The yeast diadenosine and diphosphoinositol polyphosphate phosphohydrolase DDP1 is a Nudix enzyme with pyrophosphatase activity on diphosphoinositides, dinucleotides, and polyphosphates. ScDDP1, like its human orthologs, adopts the canonical Nudix fold showing two β sheets flanked by helices. The active site lies in the crevice situated between both β sheets. The longest helix (α-1) contains the Nudix box (GX5EX7REUXEEXGU), which displays a β-loop-helix-loop structure that binds the Mg2+ ions involved in diphosphate moiety orientation and catalysis.

The most outstanding feature in the ScDDP1 overall fold is the presence of a remarkable insertion (Pro103 to Pro128) that projects out of the Nudix scaffold (named as nose from now on). This insertion is not present in the human orthologs of ScDDP1; only the S. pombe ortholog (Aps1) shows a larger insertion in this region. We have produced a ScDDP1 mutant lacking this region (Δnose mutant), which allowed us to conclude that the nose is not essential either for in vitro protein catalytic activity or folding. Similarly, on removing the protein insertion (nose) specific to yeast enzymes, the stabilization is notable (5°C), while the protein retains catalytic activity. The flexible nose has exposed hydrophobic and highly charged residues, the removal of which could result in this stabilization. The smaller DDP1 Δnose mutant stabilization gain upon polyphosphate binding suggests that part of its function could be the recognition of polyphosphates in agreement with our structural findings, which reveal that the nose residue Lys105 is close to the polyphosphate chain as well as the nose border residues Arg102 and Arg129. We have designed a nose-lacking DDP1 mutant producing an active and folded protein that depicted the outstanding influence of the nose not only in polyphosphate binding but also in all kinds of substrates. Although direct interactions of nose with the ligands have not been observed, the presence of secondary inositide molecules close to the nose suggests a possible role of this region in substrate recruitment.

> GGSMGKTADNHGPVRSETAREGRENQVYSPVTGARLVAGCICLTPDKKQVLMITSSAHKKRWIVPKGGVEKDEPNYETTAQRETWEEAGCIGKIVANLGTVEDMRPGGGPPRTEFHFYELEIENLLDKFPECHKRHRKLYSYTEAKQNLIDAKRPELLEALNRSAIIKDDK> SEVEYRAEVGQNAYLPCFYTPAAPGNLVPVC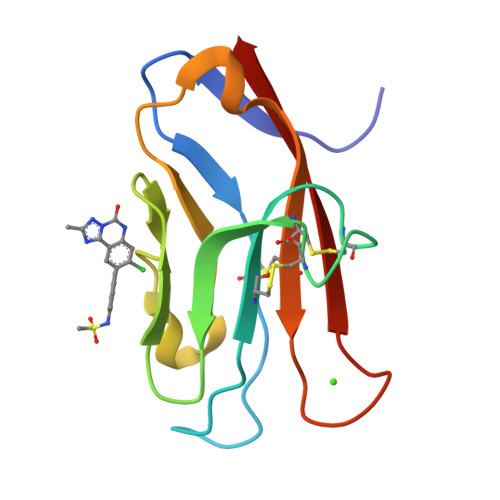WGKGACPVFECGNVVLRTDERDVNYWTSRYWLNGDFRKGDVSLTIENVTLADSGIYCCRIQIPGIMNDEKFNLKLVIK>[3x]AHCIGITDRDFIEGVHGGTWVSATLEQDKCVTVMAPDKPSLDISLETVAIDGPAEARKVCYSAVLTNVKINDKCPSTGEAHLEEENEGDNACKRTYSDRGWGNGCGLFGKGSIVACAKFTCAKSMSLFEVDQTKIQYVIRAQLHVGAKQENWNTDIKTLKFDALSGSQEAEFTGYGRATLECQVQTAVDFSNSYIAEMEKESWIVDKQWAQDLTLPWQSGSGGVWREMHHLVEFEPPHAATIKVLALGNQEGSLKTALTGAMRVTKDTNNSKLYKLHGGHVACRVKLSALTLKGTSYKICTDKMFFVKNPTDTGHGTVVMQVKVSKGAPCRIPVIVADDLTAAINKGILVTVNPIASTNDDEVLIEVNPPFGDSYIIVGRGDSRLTYQWHK

Yellow fever virus (YFV) is a re-emerging flavivirus that causes severe hepatic disease and mortality in humans. Crystallographic studies have resolved the structure of the YFV E protein and shown that its domain architecture is similar to related flaviviruses, with three N-terminal ectodomains, known as domains I (DI), II (DII) and III (DIII) and a stem anchor region known as the transmembrane domain (TM). Here we use a chimeric virus platform to resolve the first high resolution cryo-EM structures of YFV. Stark differences in particle morphology and homogeneity are observed between vaccine and virulent strains of YFV, and these are found to have significant implications on antibody recognition and neutralisation.

Exhaustive domain swap interrogation between bYFV17D and bYFVES504 revealed that DIII is a key determinant of virion icosahedral assembly and FLE mAb neutralisation. Similarly, all the chimeric virions in the bYFVES504 backbone retained their parental virus phenotype, except for bYFVES504/DIII17D, which most closely resembles the smooth phenotype of bYFV17D. Next, a cryo-EM map of bYFVES504/DIII17D was resolved to a resolution of 6.5 Å. This reconstruction displays the typical flavivirus architecture of 180 E proteins arranged in a herringbone-like pattern on the virion surface and is substantially better resolved than the bYFVES504 reconstruction. We then utilised the symmetry expanded local reconstruction method to resolve the ASU of bYFVES504/DIII17D to 3.3 Å. Similar to the bYFV17D:2C9 ASU reconstruction, M as well as the transmembrane domains of E have not been resolved. Exchange with DIII of YFV17D allowed for high resolution elucidation of the bYFVES504 virion structure in both unbound and 2C9 (E-DII mAb) bound forms, demonstrating high similarity to bYFV17D. Conversely, there was a significant increase in neutralisation of both bYFVES504/DIII17D and bYFVES504 T380R when compared with the parental bYFVES504.> SSPATSPQSTPTLVSALETIEPEVLYAGYDSSVPDSTWRIMTTLNMLGGRQVIAAVKWAKAIPGFRNLHLDDQMTLLQYSWMYLMAFALGWRSYRQSSANLLCFAPDLIINEQRMTLPDMYDQCKHMLYVSSELHRLQVSYEEYLCMKTLLLLSSVPKDGLKSQALFDAIRMTYIKELGKAIVKREGNSSQNSQRFYQLTKLLDSMHEVVENLLNYCFQTFLDKT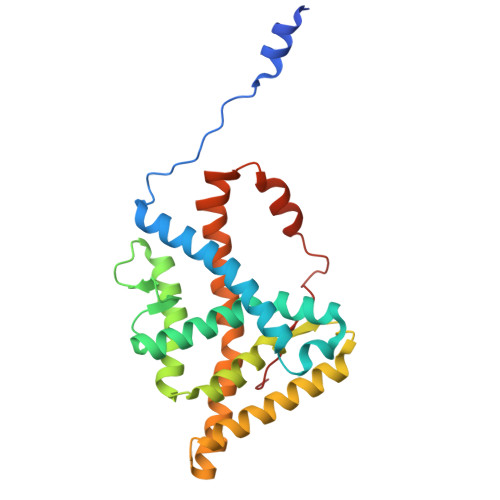MSIEFPEMLAEIITNQIPKYSNGNIKKLLFHQK> KASFTDEEDEFILDVVRKNPTRRTTHTLYDEISHYVPNHTGNSIRHRFRVYLSKRLEYVYEVDKFGKLVRDDDGNLIKTKVLPPSIKRKFSADEDYTLAIAVKKQFYRDLFQIDPDTGRSLITDEDTPTAIARRNMTMDPNHVPGSEPNFAAYRTQSRRGPIAREFFKHFAEEHAAHTENAWRDRFRKFLLAYGIDDYISYYEAEKAQNREPEPMKNLTNRPKRP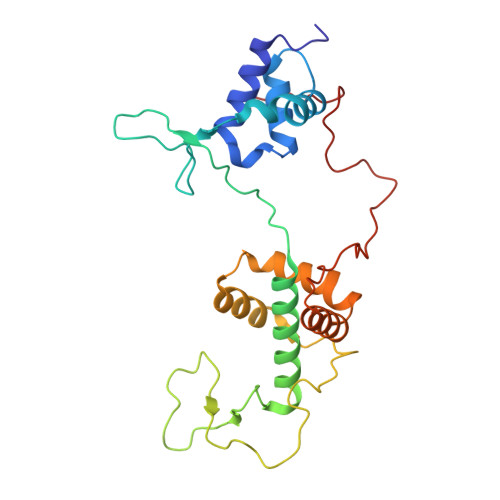GVPTPGNYNSAAKRARN> GCGTGGGCA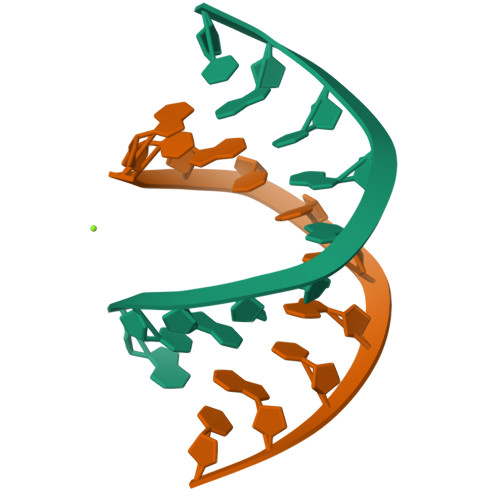C;> GTGCCCACGC> GSMAWFFGKIPRAKAEEMLSKQRHDGAFLIRESESAPGDFSLSVKFGNDVQHFKVLRDGAGKYFLWVVKFNSLNELVDYHRSTSVS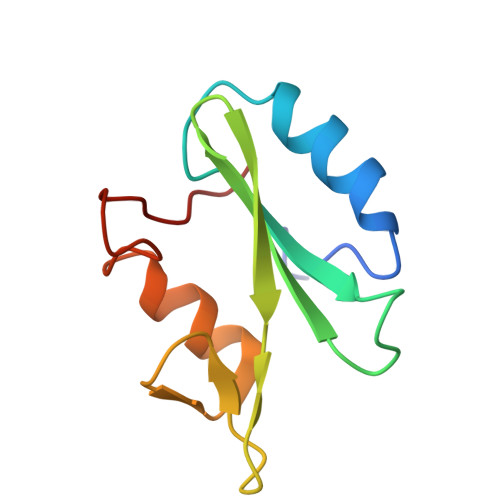RNQQIFLRDI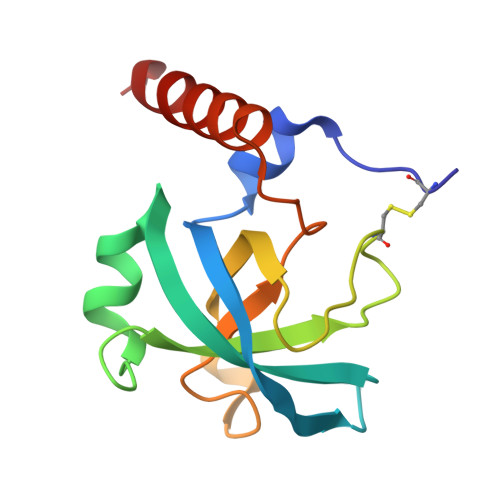> NCPERELQRREEEANVVLTGTVEEIMNVDPVHHTYSCKVRVWRYLKGKDIVTHEILLDGGNKVVIGGFGDPLICDNQVSTGDTRIFFVNPAPQYMWPAHRNELMLNSSLMRITLRNLEEVEHCVEEHRKLL> MAEVRVQLLLSRRPESVSFARSVCGLLGAGPGLGTWPIHCSLKRGRLVLSSRPFPGASARLPLQRPPFCPFAALEERPRVPGAE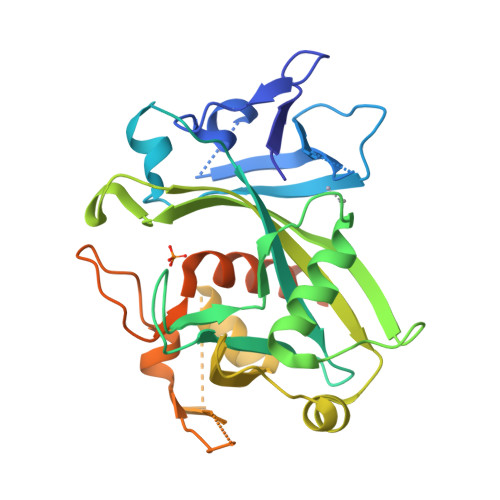LPTDRGVDLGVAVILQSSDKTVLLTRRARTLSVSPNLWVPPGGHVELEEELLDGGLRELWEESGLHLPQGQFSWVPLGLWESAYPPRLSWGLPKYHHIVLYLLVISQESQQQLQARIQPNPNEVSALMWLTPDVAAAVAAAEDGTETPGLLPQDLPPSVLAVELEEDGRARPLVLHMSTLLRMIPTMAEDKERVSTGTKFALKLWLQHLGRTPPPCKSAAYLDPGPAKEEWNMDPLPPNQGSGK> MAFSELLDLVGGLGRFQVLQTMALMVSIMWLCTQSMLENFSAAVPSHRCWAPLLDNSTAQASILGSLSPEALLAISIPPGPNQRPHQCRRFRQPQWQLLDPNATATSWSEADTEPCVDGWVYDRSIFTSTIVAKWNLVCDSHALKPMAQSIYLAGILVGAAVCGPASDRFGRRLVLTWSYLQMAVSGTAAAFAPTFPVYCLFRFLLAFAVAGVMMNTGTLLMEWTSARARPLVMTLNSLGFSFGHGLTAAVAYGVRDWTLLQLAVSVPFFLCFLYSWWLAESARWLLTTGRLDRGLQELRRVAAINGKRAVQDTLTPEVLLSAMREELSVGQAPASLGTLLRTPGLRLRTCISTLCWFAFGFTFFGLALDLQALGSNIFLLQVLIGVVDIPAKMGALLLLSRLGRRPTLAASLLLAGLCILANTLVPHEMGALRSALAVLGLGGVGAAFTCITIYSSELFPTVLRMTAVGLGQMAARGGAILGPLVRLLGVHGPWLPLLVYGTVPVLSGLAALLLPETQSLPLPDTIQDVQNQAVKKATHGTLGNSVLKSTQF

The reabsorption process of urate in the kidney by the urate transporter URAT1 plays a pivotal role in controlling serum urate levels. URAT1 (SLC22A12) is a member of the SLC22 major facilitator superfamily transporters. The cryo-EM structures show that hURAT1 has the common architecture of SLC22 family transporters, which is formed by the N-terminal domain (NTD) with an extracellular protrusion and the C-terminal domain (CTD). Structural comparison between different conformations of hURAT1 reveals the rocker-switch-like mechanism for urate transport.

Benzbromarone is a high-affinity hURAT1 inhibitor, which was clinically used for the treatment of gout. We determined the structure of hURAT1 in complex with benzbromarone to a resolution of 3.0 Å. In the presence of benzbromarone, the structure exhibits an inward-facing conformation, in which the extracellular vestibule is sealed and the intracellular vestibule is open. Benzbromarone binds at the urate-binding site. The ethyl-benzofuran group of benzbromarone is surrounded by C32, S35, M36, F241, and H245 of the NTD, and F360, F364, and F365 of the CTD. The dibromo-hydroxyphenyl group of benzbromarone forms hydrophobic interactions with F449. Moreover, the side chains of Q473 and N237 form polar interactions with the hydroxyl group and bromine atom of benzbromarone, respectively. In contrast, the N237A, F360T, and F364Y mutants maintained urate uptake activity similar to hURAT1WT, but all reduced the potency of benzbromarone to varying degrees. Notably, F360T had the most pronounced effect, highlighting the critical role of F360 in benzbromarone’s potency. Specifically, benzbromarone clashes with the side chain of F449 of the CTD, and verinurad clashes with R447 of the CTD of hURAT1 in the outward-facing conformation.>[2x]MGHHHHHHHHHHSSGHIEGRHMPFPYSIDFVESKQNEQLLKDFHGERTGFVQVGEKRWFFPSRFKQYAESLYSFEARPDDTWIVTYPRSGTTWSQEMVWLLCNELDFETAKSIPLTQRFPFLEFHLFVHDEVKAEFLKENEHDVESMK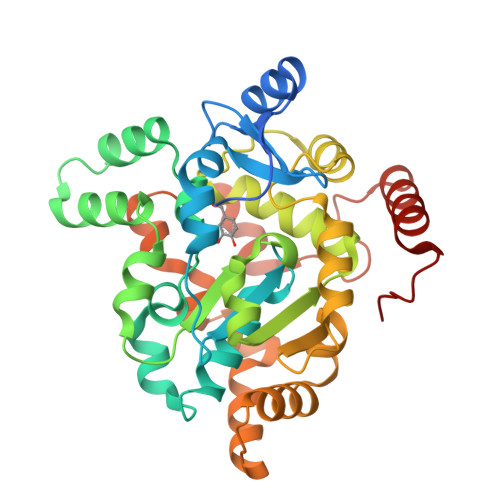FIEQLSQPAGFMLAEMKTPRFIKTHLPISLLPPSVFEQKAKIIYVARNPSDVAVSYYHLNRLYRTQGYVGDFETFYNYFEKDLTPWSPYWEHIKEGWAERDRENVLFMYYEDMKRNLPDTIRKTAAFLGKSFSDDQIDTMCTHLDIRNFRHNKSVTCEELKAVGILNSGEQGFVRNGQVRGNAEEMTDDIKRRLNEWTERNLNGTDIRFPDC>[2x]GMIPFPE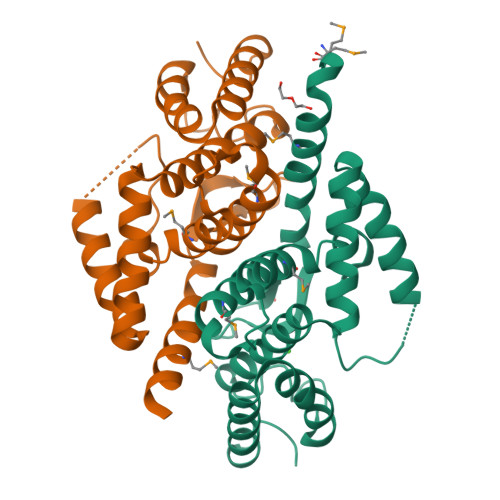SRLAAQMSFVVEIDKLKTILRQTLLTDSSRRENDAEHSWHIATMAFLLAEYADEAVQIGRVARMLLIHDIVEIDAGDTFIHDEAGNEDKEERERKAAARLFGLLPPDQAAEYSALWQEYEARETADARFADALDRLQPLLHNFETEGGTWKPHGVTRAKVDKLLPRIEAGSKRLGAYARALVDEAVRRGYLAP> MNDSSVIYRAIVTSKFRTEKMLNFYNSIGSGPDKNTIFITFGRSEPWSSNENEVGFAPPYPTDSVLGVTDMWTHMMGTVKVLPSMLDAVIPRRDWGDTRYPDPYTFRINDIVVCNSAPYNATESGAGWLVYRCLDVPDTGMCSIASLTDKDECLKLGGKWTPSARSMTPPEGRGDAEGTIEPGDGYVWEYLFEIPPDVSINRCTNEYIVVPWPEELKEDPTRWGYEDNLTWQQDDFGLIYRVKANTIRFKAYLDSVYFPEAALPGNKGFRQISIITNPLEAKAHPNDPNV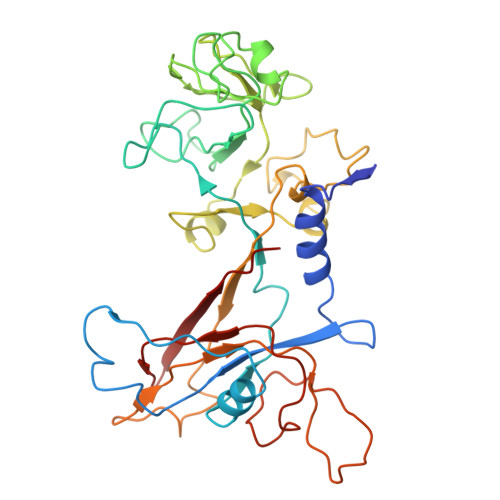KAEKDYYDPEDLMRHSGEMIYMENRPPIIMAMDQTEEINILFTF>[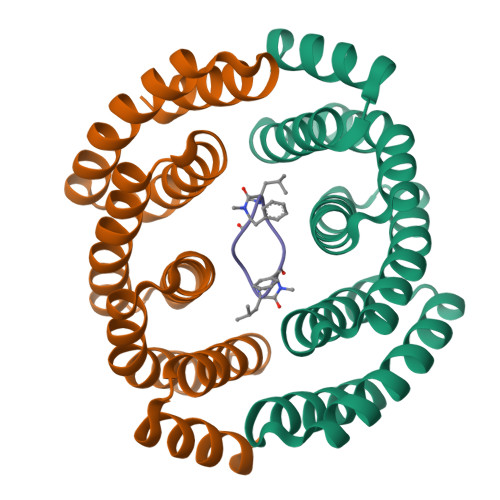2x]SMLEEIERLVLSGLLTGDKELLKKASELLKEEMEKLLEEGDLDALKKALQLAVNVADHNGDKELLAHAAEVIKRALDLALEAKDLQSAKYLASLALWIAKRAGDKELYAYLEEKIKKIIELAEEAGDRESLKILILLGIFIARDAGSEEVKAFVAEQLERLL;> PLFAPLFA Here, we discover a family of Bdellovibrio proteins that define a new subgrouping of the lysozyme superfamily and demonstrate that they possess outright specificity for deacetylated peptidoglycan. We solve the structure of family member Bd0314 (that we named DslA), revealing adaptations to the lysozyme fold that sterically restrict the active-site cleft into only accepting polymers deacetylated at the GlcNAc positions. We determine a role for DslA in B. bacteriovorus exit from the prey cell and demonstrate that exogenously added enzyme is able to prematurely liberate predators from prey bdelloplasts before completion of the predatory lifecycle. The architecture of DslA is related to, but significantly different from, other members of the lysozyme superfamily but still fulfil the inclusion criteria for the lysozyme superfamily noted by Monzingo et al. — conservation of the β-sheet floor and helices D and F, with appropriate placement of acidic catalytic residues.

Large crystals of a catalytic E154Q mutant enabled us to solve the structure via Sulfur-SAD phasing, finding two disulfides and two methionine residues, tracing residues 74–254 inclusive. The fold is comprised of seven major α-helices (A-G), several smaller 310 helices, an elongated β-hairpin (b1–2) and a smaller β-hairpin (b3-4). The fold is stabilized by disulfide bonds between C117:C253 and C182:C199. A second acidic residue, E154 projects upward from the β-sheet floor of the cleft, and its conformation is stabilized by a hydrogen bond to S166 and packing effects mediated by the hydrophobic sidechains of Y152 and F156. The pose of E154 is further influenced by interruption of main chain hydrogen-bonding: the backbone carbonyl groups of E154 and D155 point downward, not participating in β-hairpin formation. The net effect creates a bulge and allows the sidechain of E154 to face upward, directly across from E143. All four of our DslA structures (two wild-type, E143Q, E154Q) are highly similar, other than a relatively small flexation of the β1–2 hairpin in the E154Q variant. Variants E143Q and E154Q clearly fold and retain a similar active-site architecture (as judged by our high-resolution structures herein), but display no notable activity (middle), confirming their participation in catalysis. Residue E143 of the conserved ES motif would act as a general acid, protonating the equatorial linkage between MurNAc and GlcN, with E154 acting as a general base to activate water to attack the MurNAc C1 in an axial orientation. The structural equivalence of DslA E154 to the β1 secondary catalytic acid residues of goose-type lysozymes (also GH23, but with a second catalytic residue lacking in the lytic transglycosylases), v-type lysozymes and chitosanases, and our assay on the E143Q and E154Q mutants argues for an inverting hydrolytic mechanism for DslA.

> MKNTPQHKLFFVVALLLVVQILAGCKSSSSTTAGSTENSSSSTPDPDTGTTTPDPIEPEVVPPVTPPSVDSNSREVIPLWEDKVADGKAWSTHVYSALDKLGPNLLDVIPADRSLFCPKYSSLSYAQRKQYWAFVLSSMVRFESNFKTAMSYTQDFNDSNGNRVISRGLLQISIESGNAYGCGFKSTKDLHDPLQNLSCGIRILDRWVSRDGRIAGKVDGAWKGGARYWSVLRAGDKTSYKSIVSWSQNLSICK>[2x]GPMSEAVKNLVNNDLADVMFNRHSVRQFDPNVKIGRDELQKMIAEAATAPSACNLQSWHFVVVDTPEAKAKFKQAVMKFNYPQVDSASAIVFIAGDTQSHYVYRDVWN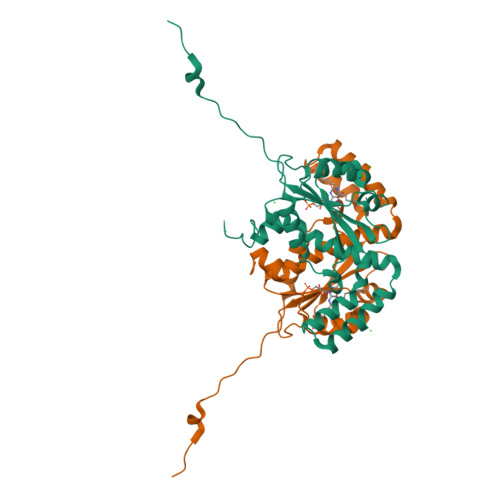KVYEDGNITKERLDQILGTFLPLYENATPDFLKFDATIDCSVVGMQLLLVARAHGYDANAFSGIDFEKMIPTLGLDPKRYVPVMGIAIGKAAQEPLHTTRYDAKTQTDFLA>[2x]MYKLVPQIDTRDCGPAVLASV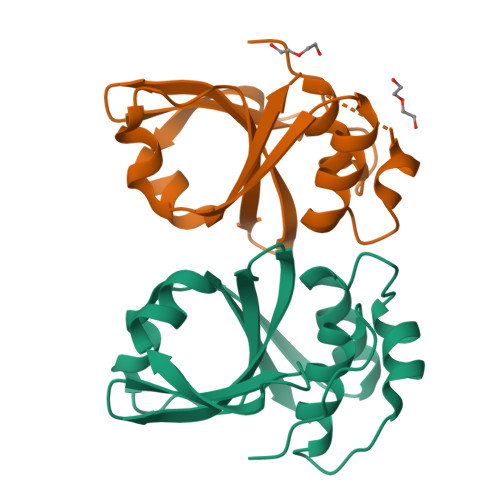AKHYGSNYSIAYLRELSKTNKQGTTALGIVEAAKKLGFETRSIKADMTLFDYNDLTYPFIVHVIKGKRLQHYYVVYGSQNNQLIIGDPDPSVKVTRMSKERFQSEWTGLAIFLAPQPNYKPHKGEHHHHHH>[2x]GC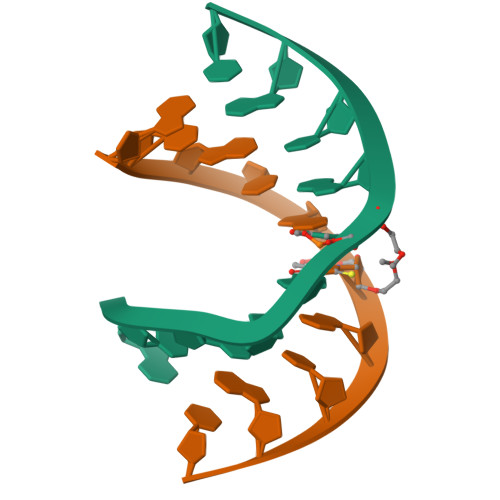GTATACGC> GSEFQNKNFRAPQSEAIGILYKL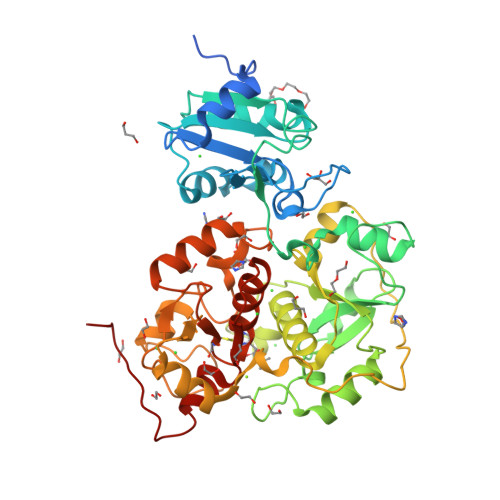IETGSKHKNMYDHTEITTDSLLALLGSEKVKIIDVRSADAYNGWRMRGEVRGGHIKGAKSLPAKWLTDPEWLNIVRFKQIRPEDAIVLYGYTPEECEQTATRFKENGYNNVSVFHRFHPDWTGNDAFPMDRLEQYNRLVPAEWVNGLISGEEIPEYDNDTFIVCHAHYRNRDAYLSGHIPGATDMDTLALESPETWNRRTPEELKKALEEHGITASTTVVLYGKFMHPDNADEFPGSAAGHIGAIRLAFIMMYAGVEDVRVLNGGYQSWTDAGFAISKDDVPKTTVPEFGAPIPSRPEFAVDIDEAKEMLQSEDSDLVCVRSYPEYIGEVSGYNYIKKKGRIPGAIFAECGSDAYHMENYRNHDHTTREYHEIEDIWAKSGIIPKKHLAFYCGTGWRGSEAWFNALLMGWPRVSVYDGGWFEWSNDPENPYETGVPK>MSLRRGIYHIENAGVPSAIDLKDGSSSDGTPIVGWQFTPDTINWHQLWLAEPIPNVADTFTLCNLFSGTYMDLYNGSSEAGTAVN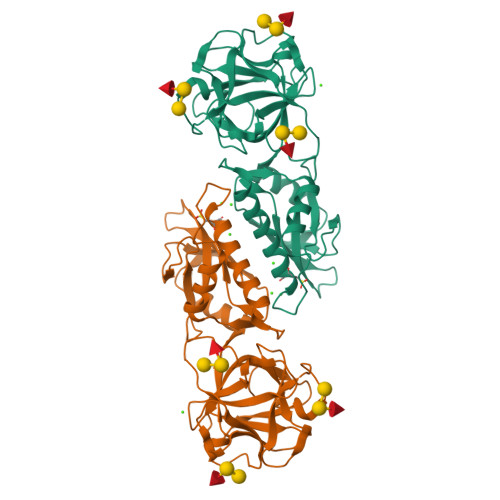GWQGTAFTTNPHQLWTIKKSSDGTSYKIQNYGSKTFVDLVNGDSSDGAKIAGWTGTWDEGNPHQKWYFNRMSVSSAEAQAAIARNPHIHGTYRGYILDGEYLVLPNATFTQIWKDSGLPGSKWREQIYDCDDFAIAMKAAVGKWGADSWKANGFAIFCGVMLGVNKAGDAAHAYNFTLTKDHADIVFFEPQNGGYLNDIGYDSYMAFY[4x]> GPANNDQDEDRINDKMKRRLAQNREAARKSRLRKKAHVQQLEESRLKLSQLEQELVRARQQGLCVRNSSDTSYLGPAGNMNSGIAAFEMEYTHWLEEQNRRVSEIRTALQAHIGDIELKMLVDSCLNHYANLFRMKADAAKADVFFLMSGMWRTSTERFFQWIGGFRPSELLNVVMPYVEPLTDQQLLEVRNLQQSSQQAEEALSQGLDKLQQGLVESIAIQIKVVESVNHG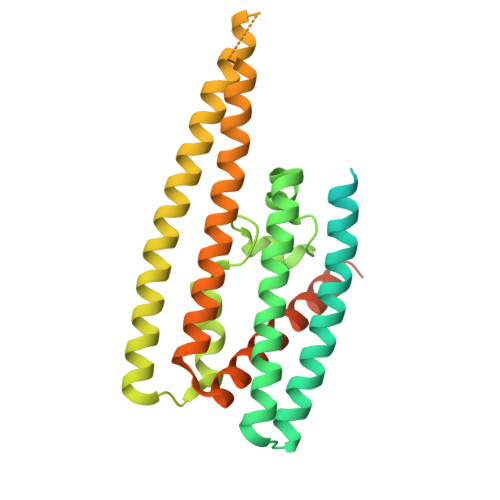APMASAMENLQALESFVNQADHLRQQTLQQMSKILTTRQAARGLLALGEYFHRLRALSSLWAARPREHTGGDYKDDDDKSSGYPYDVPDYA>GSKKIFKPEELRQALMPTLEALYRQDPESLPFRQPVDPQLLGIPDYFDIVKNPMDLSTIKRKLDTGQYQEPWQYVDDVWL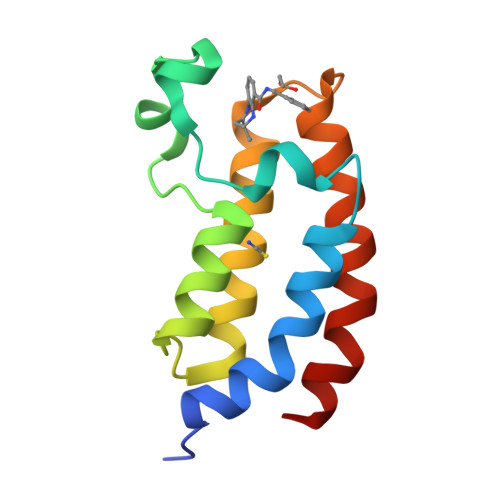MFNNAWLYNRKTSRVYKFCSKLAEVFEQEIDPVMQSLG[2x]>KPNVAIIVAALKPALGIGYKGKMPWRLRKEIRYFKDVTTRTTKPNTRNAVIMGRKTWESIPQKFRPLPDRLNIILSRSYENEIIDDNIIHASSIESSLNLVSDVERVFIIGGAEIYNELINNSLVSHLLITEIEHPSPESIEMDTFLKFPLESWTKQPKSELQKFVG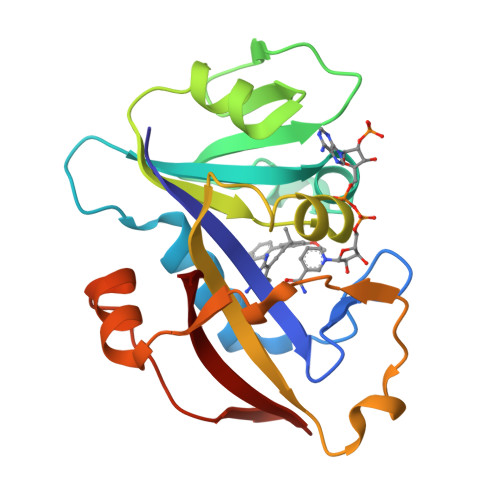DTVLEDDIKEGDFTYNYTLWTRK[2x]> MPVNQSDNNQSEVVTRSATGIKNIVYIEVNDINPLNAGSYIMDDAPFFDYVILFAANIRGVGSDATLYNNPNVQYILDHKDTLIKPLQDKGIKVLLGLLGDHTGLGFANMNSAQTEQFATAVANAVSQYGLDGVDFADAWAEYGRNGYPSGSTGSFSNLITALHNKMPGKTITVFNYGYTSELTGVNSYIDYGIYAFFNSPSWSTGFGMPNSKFAPYTINLNSAPSAASAQLYSGQVASKGYGAIGYYDLRANNIVSVLNGVAKGAFKSTCTYDGNSYPKNY

The genomes of Bacteroidales contain genes encoding glycan-degrading apparatuses that typically co-localize in discrete clusters known as polysaccharide utilization loci (PULs). B. thetaiotaomicron contains almost 300 different GHs belonging to 60 different GH families, and secretes at least six mannosyl-glycoprotein endo-β-N-acetylglucosaminidases (ENGases, endoglycosidase hereafter) that hydrolyze the chitobiose core of asparagine-linked, or N-linked, glycans (EC 3.2.1.96). Here, we discover an ENGase from the GH18 family in B. thetaiotaomicron, BT1285, encoded in a distinct PUL with its own repertoire of proteins for catabolism of the same HM N-glycan substrate as that of BT3987. Altogether, our data suggest that human gut microbes employ evolutionary strategies to express distinct ENGases in order to optimally metabolize the same N-glycan substrate in the gastroinstestinal tract.

To better understand the molecular mechanism by which BT1285 specifically hydrolyzes N-glycans, we solved the crystal structure of a catalytically inactive variant of BT1285 (BT1285D161A-E163A; hereafter BT1285i) in complex with the Man9GlcNAc2 substrate at 1.9 Å resolution. We observed no substantial conformational changes in the protein backbone for the unliganded and glycan-bound forms of BT1285 (r.m.s.d. of 0.4 Å for 271 residues). While both BT1285i and BT3987i inactive ENGases bind to the Man5 oligomannose on RNAseB, BT1285i exhibited a 1000-fold higher binding affinity than BT3987i (KDs of 3.5 nM versus 4.3 μM). Therefore, glycan accessibility clearly plays a role in these binding events, as the affinity of BT1285i for the exposed glycan on RNAseB was 12-fold higher than for the constrained glycans on IgG (KDs of 3.5 nM versus 42 nM). By using size exclusion chromatography (SEC) we determined that BT1285i forms a stable complex with either Fc-IgG1-HM and IgG1-HM, but not with IgG-CT as expected. SDS-PAGE analysis of the SEC fractions indicated the formation of a 2:1 BT1285i:Fc-HM highly stable complex. Moreover, inactive mutants of ENGases generated in this work (e.g. BT1285i) that recognize different HM N-glycans with such high affinity could potentially be used as artificial lectins with high specificity for targeting tumor-associated HM N-glycans molecules, potentially aiding cancer treatment.> LNEHTAGDTTKSPYTIYAGLGFAVQESCYYCHGNGGKGTTEGLIFGVPDFTSTEFQSSMTD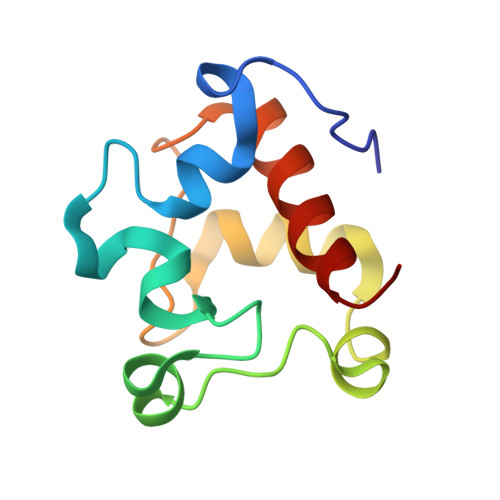KQIIDHINKGKGKCPSYQGKMSPEMIEKMAGVVRNFAVK>METIQELILSEENKTNIAVLNLGTNDRRNAVLILETALHLVEKYLGKIINTSYLYETVPEYIVLDKKESCEKINKDCRIYDVNYINELMQNLEESKYEENKELIDKCEEYETFLKNGKVDNSILKEVNVENYLLECNNIIVKNDEIMKNNLSKYKDKYYTSYFYNLTVVVKTFVNDPLSMLVVIKYIEELMKRENVKEKEKFENRIIDIDILFFNDFTIFMKNIKLEKNMIYKILSKYIHLERDIKNGNDNMSKVNMDKDINLNNNNNIKKKNNNDIDCDCVDQKMNNHVNNKNYINSFRDPQEIINNMVDNIEFLSIPHVYTTHRYSILLCLNDMIPEYKHNVLNNTIRCLYNKYVSRMKEQYNINIKENNKRIYVLKDRISYLKEKTNIVGILNVNYDSFSDGGIFVEPKRAVQRMFEMINEGASVIDIGGESSAPFVIPNPKISERDLVVPVLQLFQKEWNDIKNKIVKCDAKPIISIDTINYNVFKECVDNDLVDILNDISACTNNPEIIKLLKKKNKFYSVVLMHKRGNPHTMDKLTNYDNLVYDIKNYLEQRLNFLVLNGIPRYRILFDIGLGFAKKHDQSIKLLQNIHVYDEYPLFIGYSRKRFIAHCMNDQNVVINTQQKLHDEQQNENKNIVDKSHNWMFQMNYMRKDKDQLLYQKNICGGLAIASYSYYKKVDLIRVHDVLETKSVLDVLTK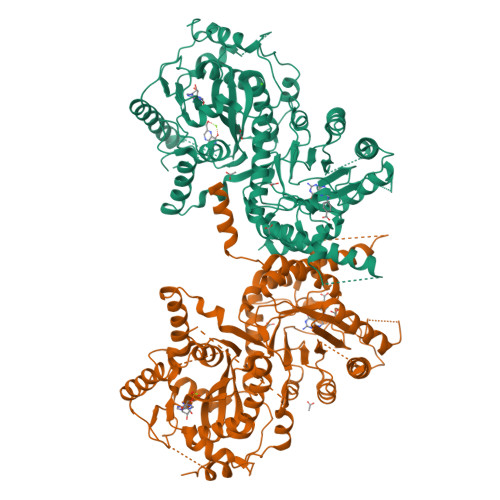IDQVKDPNSSSVDKLAAALEHHHHHH[2x]>[4x]VPLSRTVRCTCISISNQPVNPRSLEKLEIIPASQFCPRVEIIATMKKKGE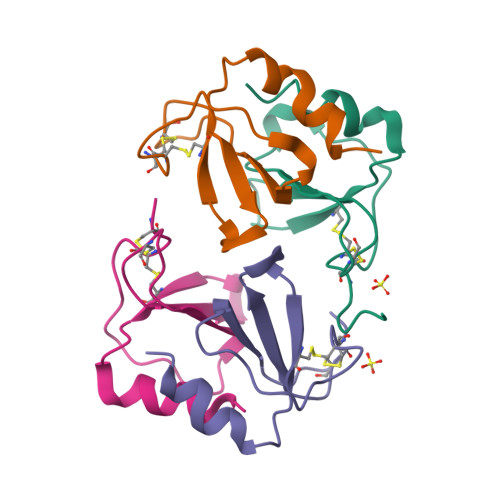KRCLNPESKAIKNLLKAVSKEMSKRSP>MAFPKRLEYGGHALVWSGDWSAAGARKAIAGAARAGYDYIEIALLDPWQIDVALTKDLLQEYNLRAHASLGLSAATDVTSTDPAIVAKGDELLRKATDVLYALGGSELCGVIYCALGKYPGPAS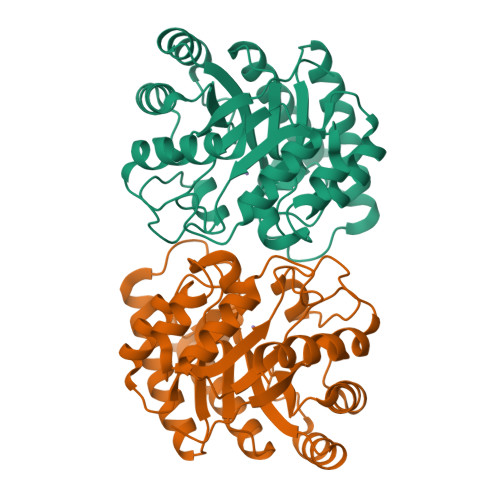RENRANSVAAMQRLADYAADKGINIDLEVVNRYETNIMNTGLEGLAFLDEVNRPNAFLHLDTYHMNIEENGMAKSVLAAGDRLGYVHIGESHRGYLGTGNVDFASFFAALKQIDYRGPITFESFSSEIVDPKLSNTLCVWRNLWHDSDDLAGKALEFIKQRYGSHHHHHH[2x]5'-O-[(R)-hydroxy{[(4R,8S)-4,6,8-trihydroxy-2,4,6,8-tetraoxo-1,3,5,7,2lambda~5~,4lambda~5~,6lambda~5~,8lambda~5~-tetroxatetraphosphocan-2-yl]oxy}phosphoryl]adenosine | C10 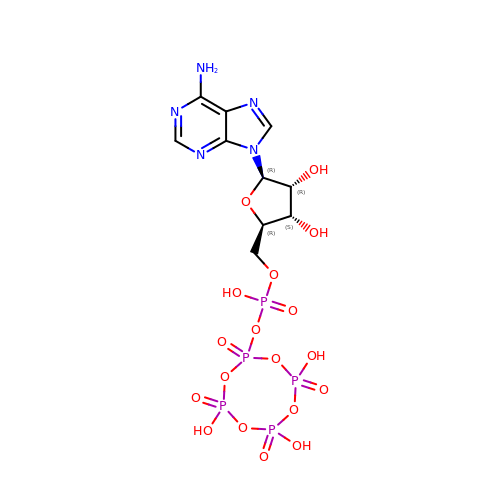H16 N5 O18 P5 | WWRLCZMRKAWYHG-KQYNXXCUSA-N>[2x]MAGHTDNEITIAAPMELVWNMTNDIEKWPGLFSEYASV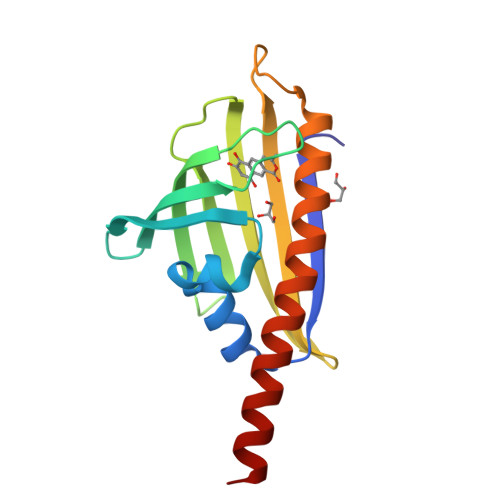EVLGRDDDKVTFRLTMHPDADGKVWSWVSERVADPVTRTVRAQRVETGPFQYMNIVWEYAETAEGTVMRWTQDFAMKPDAPVDDAWMTDNINRNSRTQMALIRDRIEQAAGERRTASVLAD>MPDQRQTRFAHITKAHPCFNEKLHDRVGRVHVPIAPRCNIHCKFCTRDINECERRPGVTGRLMTADDAIKHVEKVKEEMPISVIGVAGPGDALANEETFEFFKKASKKFPDLLKCMSTNGLLLPDRADELAELGINTVTVTVNAVDPEIGEKIYSFVVYKDKVYHGREAFEVLSRNQLEGIEKLAERGIIVKVNSVLIPGLNDEHIVDIAREVKKRGASLMNIIPLIPMGEMKDYPRPTCEQIERVRNEVEKIIPVFRACTQCRADAYGIPGKKEADKHLDMTPASHY[2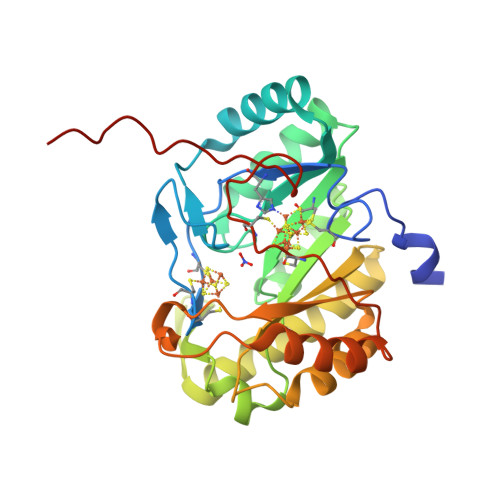x]The A. salmonicida LFI1238 genome harbors genes encoding two family AA10 LPMOs (AsLPMO10A, AsLPMO10B) and one chitinase GH18 (AsChi18A). LPMOs were discovered in 2010, and thus represent a recent addition to the chitin degradation machinery. These copper-dependent, redox enzymes cleave chitin chains by an oxidative reaction and synergize with chitinases in chitin degradation reactions. Can it be that the two LPMOs have different functions? Both A. salmonicida LPMOs cleave chitin chains by oxidation and contribute to chitin catabolism. In conclusion, we have shown that the LPMOs of A. salmonicida may be moonlighting enzymes that not only contribute to chitin catabolism, but also play a role in the pathogenicity of the bacterium in the invasive phase of CWV in Atlantic salmon.

A structural investigation of AsLPMO10B was initiated to find a rationale for its apparent role as a facilitator during host invasion. AsLPMO10B carries the canonical fibronectin-like/immunoglobulin-like β-sandwich core structure found in other LPMOs, consisting of seven β-strands arranged as two juxtaposing β-sheets. The β-sandwich supports the histidine brace catalytic motif (His26, His136) and the putative co-substrate coordinating amino acid (Glu206), which shows conformational heterogeneity and was modeled in two alternative conformations. The histidine brace is loaded with a copper ion, as confirmed by anomalous scattering, an expected consequence of the sample preparation process. Copper shows an incomplete square planar coordination, hinting at the presence of Cu (I) at the metal-binding site. The latter is likely a consequence of the well-documented photoreduction of Cu (II) during X-ray data collection. We also observe electron density “above” the copper site, where the putative ligand would bind, which may represent a citrate molecule from the buffer. In particular, the distinctive loop 2 (L2) of subcluster 2 is conserved in AsLPMO10B. Tma12 has been proven to shield its host from predators by exerting an entomotoxic activity. Their structural superposition reveals a possible site for AsLMPO10B O-linked glycosylation at Thr166, matching the N-linked glycosylation of Tma12 at Asn158. Moreover, we note the structural similarity of the AsLPMO10B AA10 domain with the chitin-active AA10-domain of viral fusolin, an LPMO that strongly enhances the infectivity of entomopoxviruses, indicating shared structural features that enable an LPMO to enhance the virulence of a pathogen.

> MTNTIKINSLTIAFVGALSSMGVQAHGWVEYPSARQNTCYLDGGFWDNTIPNQACQSAFDESGAFPFVQRNEVAANVPNYKDMAHVQAIVRDGNLCSAGDKAKSGLNMGSTHWQKTAITLDENNQLELVFNATAPHNPSYWQFYLSNVNYDPTVPLTWGDLDVVDTAGDIIVGDDKKYRIKITLPADRADSAVLYTRWQREDAAGEGFYNCSDIAFDGAGTTPPGPIDPVEPPPQYSDLGYYIGQGFGPVESGDSVRFRTFDATGAETTDISLAITVNNTATWSAELAGQFNQLKNKAWFIGIWHQEMNHYMYDTINIYANRVFAPKANLSYQLSLIKADITPPVEPPVEPTNQWDKNNAYQARESVTHQGGTWVAQWWTKGEEPGKTGEWGVWR>KTLVYCSEGSPEGFNPQLFTSGTTYDASSVPLYNRLVEFKIGTTEVIPGLAEKWEVSEDGKTYTFHLRKGVKWHDNKEFKPTRELNADDVVFSFDRQKNAQNPYHKVSGGSYEYFEGMGLPELISEVKKVDDNTVQFVLTRPEAPFLADLAMDFASILSKEYADAMMKAGTPEKLDLNPIGTGPFQLQQYQKDSRIRYKAFDGYWGTKPQIDTLVFSITPDASVRYAKLQKNECQVMPYPNPADIARMKQDKSINLMEMPGLNVGYLSYNVQKKPLDDVKVRQALTYAVNKDAIIKAVYQGAGVSAKNLIPPTMWGYNDDVQDYTYDPEKAKALLKEAGLEKGFSIDLWAMPVQRPYNPNARRMAEMIQADWAKVGVQAKIVTYEWGEYLKRAKDGEHQTVMMGWTGDNGDPDNFFATLFSCAASEQGSNYSKWCYKPFEDLIQPARATDDHNKRVELYKQAQVVMHDQAPALIIAHSTVFEPVRK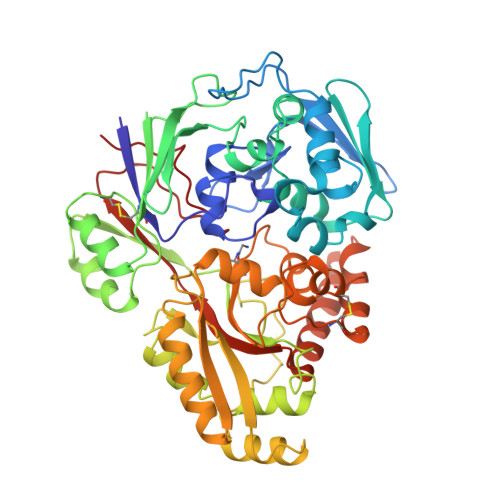EVKGYVVDPLGKHHFENVSIE[4x]>[2x]ARKCSLTGKWTNDLGSNMTIGAVNSRGEFTGTYTTAVTATSNEIKES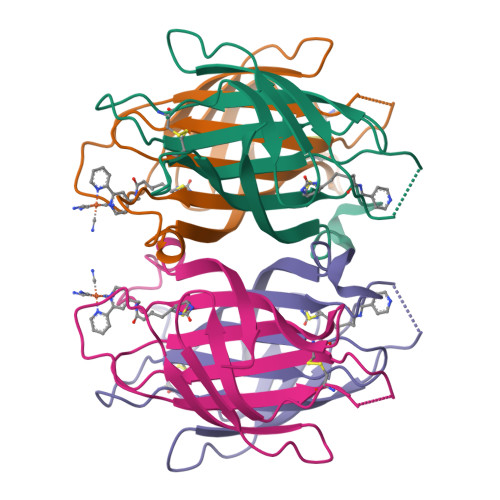PLHGTENTINKRTQPTFGFTVNWKFSESTTVFTGQCFIDRNGKEVLKTMWLLRSSVNDIGDDWKATRVGINIFTRLRTQKE>[4x]HHHHHHAGAEGALIRFYVEIEEPEKFLNCVPEELKETLLKEKRIYIDVFTTRPDTVFGATFVVLAPEHPLVPVLACIGERLGNAC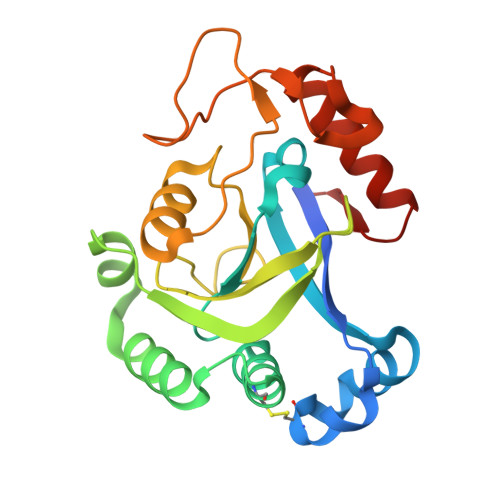YSDVENFVEKMKKMSTRERTMEEDKEGVFLGVYATNPANGEKIPVWSANYVLYEYGTGAIMCVPAHDQRDWEFAKKYDLPIKVVVKPEGAWDFEKGAYEGKGTLVNSDGFDGLDSETAKRKITEWLQDRGLGEKKV>[4x]GKLPPVYPVTVPILGHIIQFGKSPLGFMQECKRQLKSGIFTINIVGKRVTIVGDPHEHSRFFLPRNEVLSPREVYSFMVPVFGEGVAYAAPYPRMREQLNFLAEELTIAKFQNFVP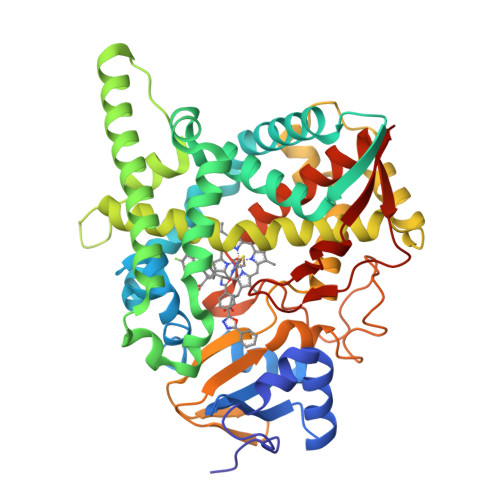AIQHEVRKFMAANWDKDEGEINLLEDCSTMIINTACQCLFGEDLRKRLDARRFAQLLAKMESSLIPAAVFLPILLKLPLPQSARCHEARTELQKILSEIIIARKEEEVNKDSSTSDLLSGLLSAVYRDGTPMSLHEVCGMIVAAMFAGQHTSSITTTWSMLHLMHPANVKHLEALRKEIEEFPAQLNYNNVMDEMPFAERCARESIRRDPPLLMLMRKVMADVKVGSYVVPKGDIIACSPLLSHHDEEAFPEPRRWDPERDEKVEGAFIGFGAGVHKCIGQKFGLLQVKTILATAFRSYDFQLLRDEVPDPDYHTMVVGPTASQCRVKYIRR> MESTALQQAFDTCQNNKAAWLQRKNELAAAEQEYLRLLSGEGRNVSRLDELRNIIEVRKWQVNQAAGRYIRSHEAVQHISIRDRLNDFMQQHGTALAAALAPELMGYSELTAIARNCAI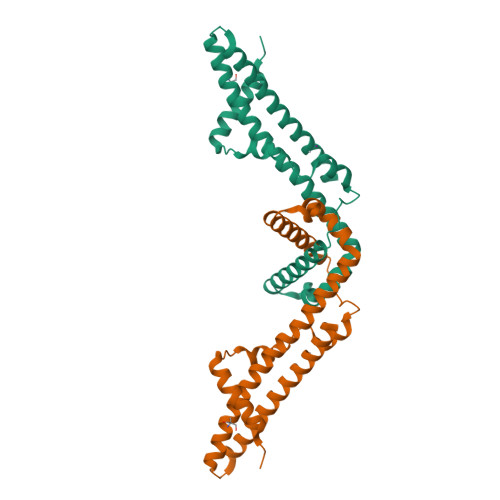QRATDALREALLSWLAKGEKINYSAQDSDILTTIGFRPDVASVDDSREKFTPAQNMIFSRKSAQLASRQSV>GSHMDYIKKAIWGPDPKEQQRRIRSVLRKNGRNIEKSLRELTVLQNKTQQLIKKSAKKNDVRTVRLYAKELYQINKQYDRMYTSRAQLDSVRMKIDEAIRMNTLSNQMADSAGLMREVNSLVRLPQLRNTMIELEKELMKSGIISEMVD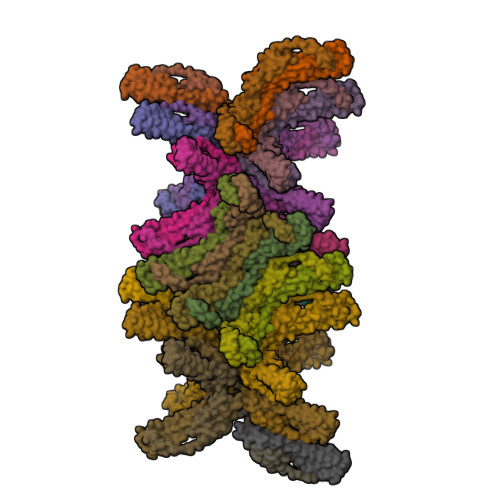DTMESVGDVGEEMDEAVDEEVNKIVEQYTNEKFKNVDQVPTVELAANEEEQEIPDEKVDEEADRMVNEMRERLRALQN[4x]> GSMAELEHLAQNISKSHLETCQYLREELQQITWQTFLQEEIENYQNKQREVMWQLCAIKITEAIQYVVEFAKRIDGFMELCQNDQIVLLKAGSLEVVFIRMCRAFDSQNNTVYFDGKYASPDVFKSL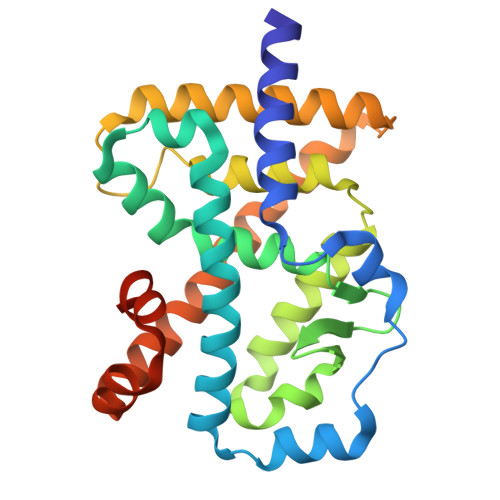GCEDFISFVFEFGKSLCSMHLTEDEIALFSAFVLMSADRSWLQEKVKIEKLQQKIQLALQHVLQKNHREDGILTKLICKVSTLRALCGRHTEKLMAFKAIYPDIVRLHFPPLYKELFTSEFEPAMQIDG> GPAMKHITVFKTYISPWERAMGVDPQQKMELGIDLLAYGAKAELPK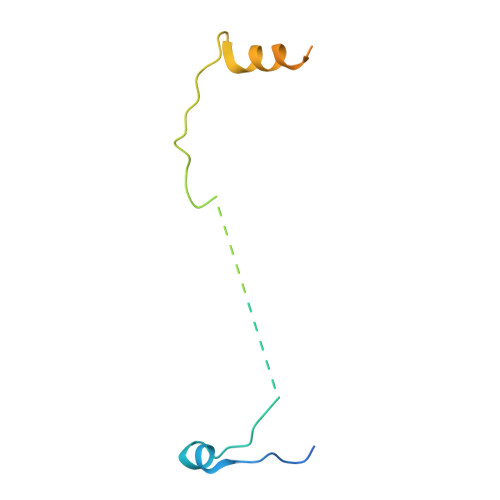YKSFNRTAMPYGGYEKASKRMTFQMPKFDLGPLLSEPLVLYNQNLS> SHMQSRELKTVSADCKKEAIEKCAQWVVRDCRPFSAVSGSGFIDMI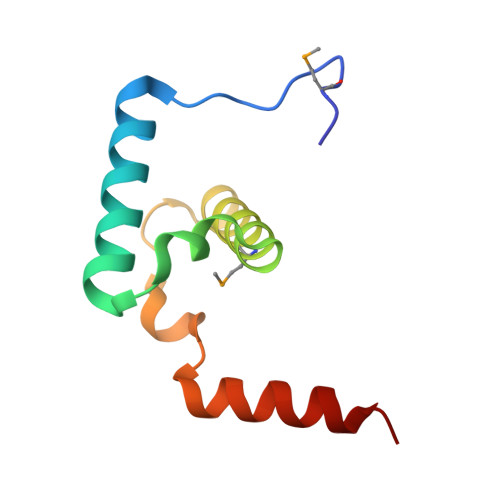KFFIKVGAEYGDHVNVEELLPSPITLSRKVTSDAKEKA> VEADTFALYALTEAQAGRSGRAKAVARLSDLLSTDPLGRLTEVEELLRAHAPTAADFARLFEACAERLTRALAEDRISRMQVTLAYSALQMALRRIHHLPDPQKSVGAVLVAGVPGHKPILEAALAAEMLRAVGWSTSVVH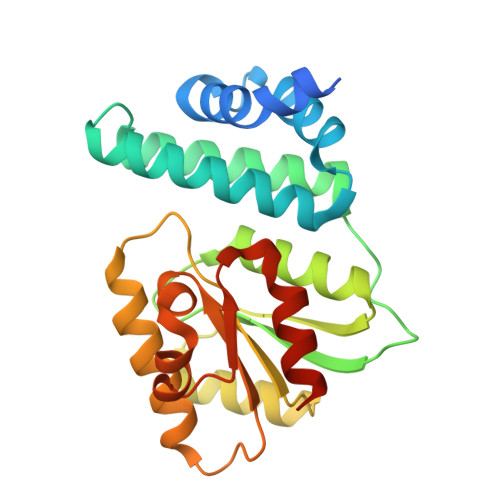PESVAALAARLKTSRTSTLVVAPSLLEGTEQEADTLRFVSALRARTDLPGLSILVGGRLAQLPPSKLKDSGADAGFAHLALLPAALARVASSAHHHHHH N-[(biphenyl-4-ylcarbonyl)carbamoyl]-beta-D-glucopyranosylamine 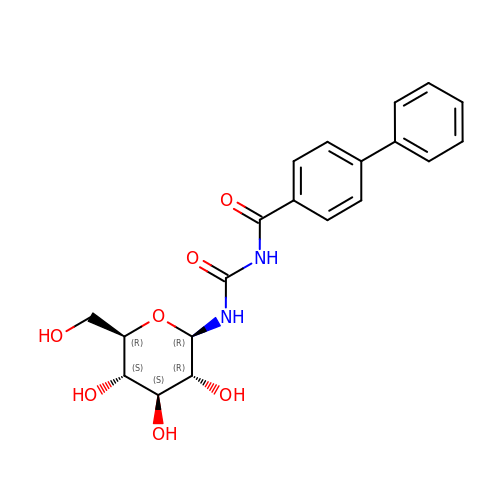| C20 H22 N2 O7 | ZINVIKWRSBKXJV-OGJJZOIMSA-N3-tert-butyl-N-[(2S)-1-(2-cyano-1,2-dimethylhydrazinyl)-4-methyl-1-oxopentan-2-yl]-1-methyl-1H-pyrazole-5-carboxamide 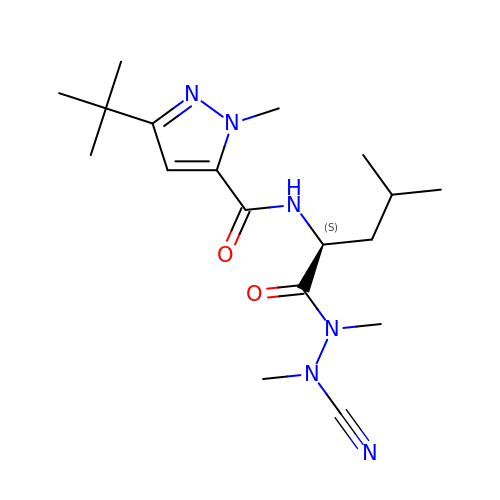(non-preferred name) | C18 H30 N6 O2 | BTSJGBRRCQOXFA-ZDUSSCGKSA-N>VDFKLSPSQLEARRHAQAFANTVLTKASAEYSTQKDQLSRFQATRPFYREAVRHGLIKAQVPIPLGGTMESLVHESIILEELFAVEPATSITIVATALGLMPVILCDSPSLQEKFLKPFISGEGEPLASLMHSEPNGTANWLQKGGPGLQTTARKVGNEWVISGEKLWPSNSGGWDYKGADLACVVCRVSDDPSKPQDPNVDPATQIAVLLVTRETIANNKKDAYQILGEPELAGHITTSGPHTRFTEFHVPHENLLCTPGLKAQGLVETAFAMAAALVGAMAIGTARAAFEEALVFAKSDTRGGSKHIIEHQSVADKLIDCKIRLETSRLLVWKAVTTLEDEALEWKVKLEMAMQTKIYTTDVAVECVIDAMKAVGMKSYAKDMSFPRLLNEVMCYPLFDGGNI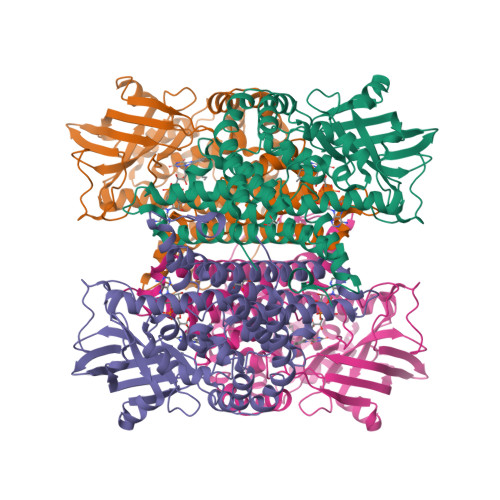GLRRRQMQRVMALEDYEPWAATYGSSKVDKSRL[4x]> MDIEDERLEELDERAESVVQLGDEVVLGTAEQELKQAPGVSIITAEDIRKRPPVNDLSEIIRTMPGVNLTGNSSSGQRGNNRQIDIRGMGPENTLILVDGKPVSSRNSVRYGWRGERDTRGDSNWVPPEEVERIEVLRGPAAARYGSGAAGGVVNIITKRPTDRLRGSMTVFTNIPESSKDG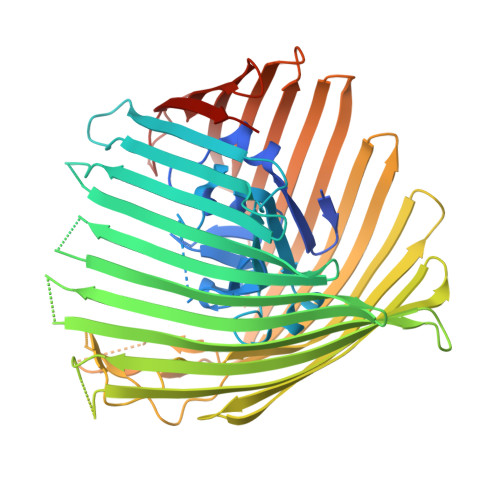ATRRANFSLSGPLTEALSFRAYGSANKTDSDDTDINLGHTVNPSRTVAGREGVRNRDLSGMLSWQVTPDQVVDFEAGFSRQGNIYAGDTQNNNGTANTQGLADDGAETNRMYRENYAITHNGTWSFGTSRFVAQYDSTRNNRLEEGLAGSVEGQIGADRSFSASKLENYRLSGELNLPLHALFEQVLTVGAEWNKETLNDPSSLKQGFVGSDSLPGTPAAGSRSPKSKAEIRALYVEDNIELRPGTMLTPGLRLDDHSDFGLNWSPSLNASQTLGEYFTVKAGIARAFKAPNLYQSNPNYLLYTRGNGCPIQTSSGGCYLVGNENLDAETSVNKELGIEFRRDGWVAGLTYFRNDYKNKIVAPLDVMGQTGTGNNILQWSNAKKAVVEGLEGNLLVPLHEDLSWSTNLTYMLQSKDKDTGNPLSVIPEYTLNSTLDWQASERLSTQLTSTIYGRQEPPKHGTSRNTPVVSRKEVGTYGIWGVSAGYTFSENLSVRGGVSNLFDKRLYRQGNSFDAGAATYNEPGRAYYVSMTTSFLSHHHHHH>[6x]NYIKPTKVNKNENGVVIDDKTVLAGSTNYYELTWDLDQYKNDRSSADTIQKGFYYVDDYPEEALELRQDLVKITDANGNEVTGVSVDNYTSLEAAPQEIRDVLSKAGIRPKGAFQIFRADNPREFYDTYVKTGIDLKIV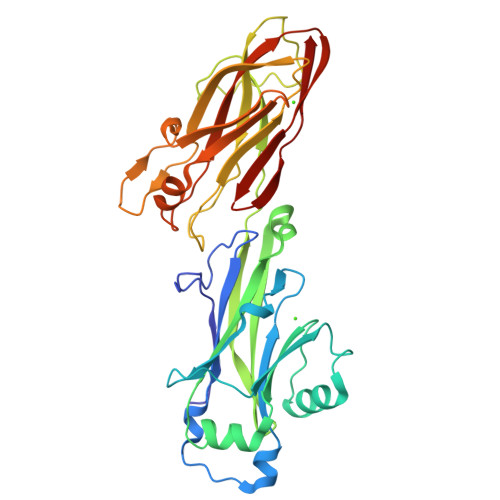SPMVVKKQMGQTGGSYENQAYQIDFGNGYASNIVINNVPKINPKKDVTLTLDPADTNNVDGQTIPLNTVFNYRLIGGIIPANHSEELFEYNFYDDYDQTGDHYTGQYKVFAKVDIILKNGVIIKSGTELTQYTTAEVDTTKGAITIKFKEAFLRSVSIDSAFQAESYIQMKRIAVGTFENTYINTVNGVTYSSNTVKTTT> APITAYAQQTRGLLGCIITSLTGRDKNQVEGEVQIVSTATQTFLATCINGVCWT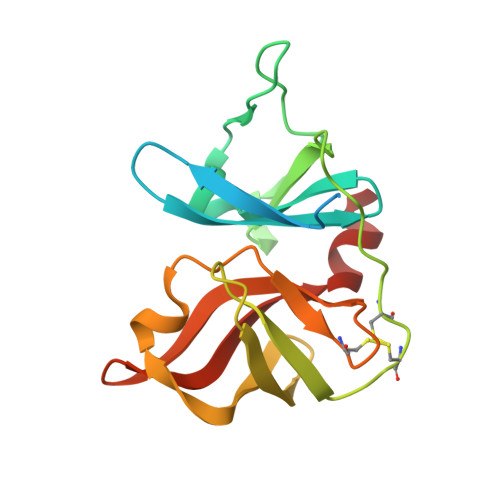VYHGAGTRTIASPKGPVIQMYTNVDQDLVGWPAPQGSRSLTPCTCGSSDLYLVTRHADVIPVRRRGDSRGSLLSPRPISYLKGSSGGPLLCPAGHAVGLFRAAVCTRGVAKAVDFIPVENLETTMRS> ASSQLIPNISPDSFTVA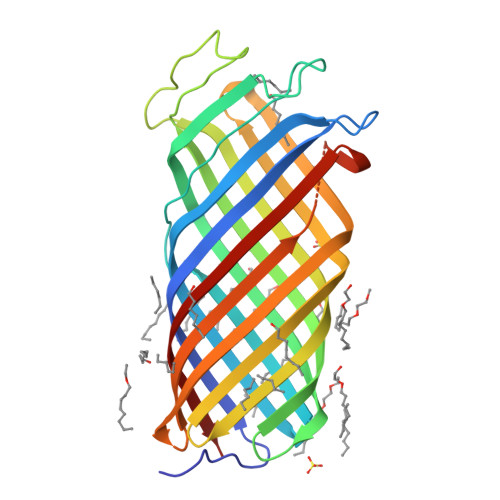ASTGMLSGKSHEMLYDAETGRKISQLDWKIKNVAILKGDISWDPYSFLTLNARGWTSLASGSGNMDDYDWMNENQSEWTDHSSHPATNVNHANEYDLNVKGWLLQDENYKAGITAGYQETRFSWTATGGSYSYNNGAYTGNFPKGVRVIGYNQRFSMPYIGLAGQYRINDFELNALFKFSDWVRAHDNDEHYMRDLTFREKTSGSRYYGTVINAGYYVTPNAKVFAEFTYSKYDEGKGGTQTIDKNSGDSVSIGGDAAGISNKNYTVTAGLQYRFG> F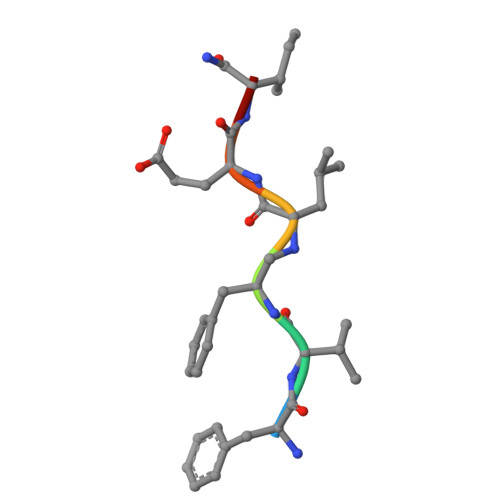VFLEIX(2R,3S)-2,3-dihydroxy-3-(1H-imidazol-5-yl)propyl dihydrogen phosphate | C6 H11 N2 O6 P | 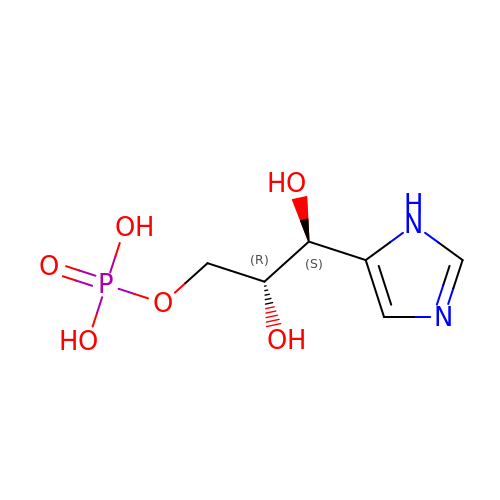HFYBTHCYPKEDQQ-RITPCOANSA-N> MKKRLTESQFQEAIQGLEVGQQTIEIARGVLVDGKPQATFATSLGLTRGAVSQAVHRVWAAFEDKNLPEGYARVTAVLPEHQ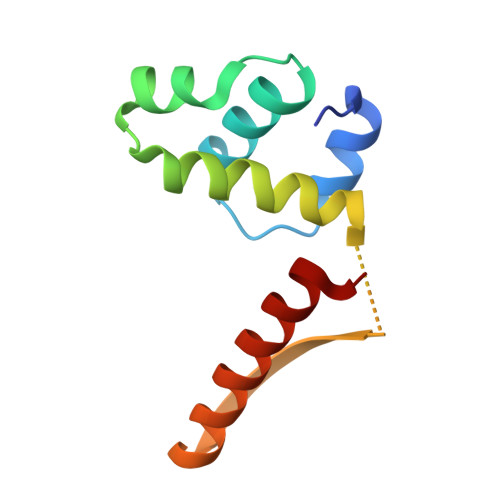AYIVRKWEADAKKKQETKR>SMFDLTGRKALVTGATGGLGEAIARALHAQGAIVGLHGTREEKLKELAAELGERIFVFPANLSDREAVKALGQKAEEEMGGVDILVNNAGITRDGLFVRMSDEDWDAVLTVNLTSVFNLTRELTHPM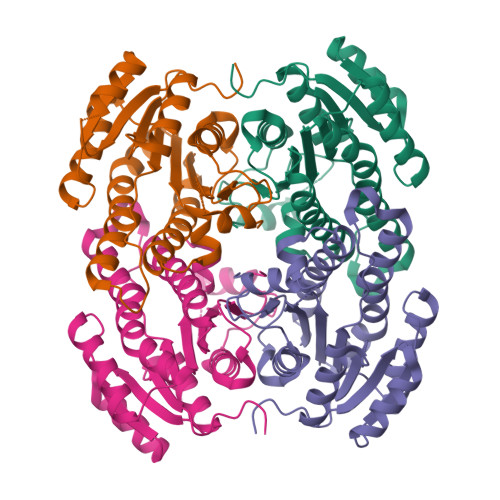MRRRNGRIINITSIVGVTGNPGQANYCASKAGLIGFSKSLAQEIASRNVTVNCIAPGFIESAMTGKLNEKQKDAIMGNIPMKRMGVGADIAAAVVYLASDEAAYVTGQTLHVNGGMAMI[4x]In these experiments, bacterial proteins with different functions were investigated. Microcrystals of photoactive yellow protein (PYP), a blue-light photoreceptor from Halorhodospira halophila, were used to explore the capability of microsecond X-ray pulses. A nitrite-reducing enzyme, cytochrome c nitrite reductase (ccNiR) from Shewanella oneidensis, was exploited to investigate potential secondary radiation damage, caused by 90 µs pulses, at heme centers. Finally, a first TR-SSX experiment was performed on the photosensory core module (PCM) of a bacterial phytochrome from the nonphotosynthetic myxobacterium Stigmatella aurantiaca.

Phytochromes are red/far-red light receptor enzymes that were originally discovered in plants, with homologs in bacteria and fungi. BphPs share a typical domain architecture comprising three conserved domains (PAS–GAF–PHY) known as the photosensory core module (PCM) and a C-terminal effector domain with enzymatic activity, usually a histidine kinase (HisK). BphPs sense red/far-red light and display a reversible photocycle triggered by the Z-to-E isomerization of a central chromophore, biliverdin (BV). This isomerization results in the formation of distinct states called Pr and Pfr (red and far-red light-absorbing states, respectively). Most notable is the conformational change of a stretch of amino-acid residues called the sensory tongue that transitions from a β-strand in the Pr state to a an α-helical conformation in the Pfr state. S. aurantiaca harbors two BphPs, SaBphP1 and SaBphP2, that bind BV and share similar domain compositions. Full-length phytochromes are challenging to crystallize, but the PCM, lacking the effector domain, forms crystals that diffract to 2 Å resolution and beyond. In the Pr state, Phe460 is buried close to the hydrophobic environment of ring D, stabilizing the Pr state.

>[2x]MPPSVSELDLSQCDREPIHLLGGIQSHGVLLAFRGPDRLLEVVSANAQALLGRPPETLLGQPVGRVLPAEVLAQWEPLVARGSVRVVLPAGAYRALLHESDGLTVLELEPAELQPGMEETALEVVRRLVSPLAGVKGTQALLQTAADTVRALTGFDRVMVYRFDADWHGEVLAESKRGGMDGFLGMHFPATDIPVQARALYTRNPLRLIADARARPVPLLPPVVPALGRPLDLSNSALRSVSPVHLEYLRNMGVGASFSLSLLKEGVLWGLIACHHLEPLHISHERRRACEVLTQLLALQLSAEERAAEASEDAHRAALLGQLATAMGEGGTLEEVLEKESERVLALTGAAGVALLLGEEPLLVGCTPAQDEVEALVAWLATQPFQTSFHTDRLGTVYPPLAARADVAAGILAVRLAPAAARFAIWFRPEVARTISWAGNPRKPAEPEPGHQRLHPRGSFQAWEETVRDTSLPWKRADLGAAEGFRGALV>MVLYFIGLGLYDERDITVKGLEIAKKCDYVFAEFYTSLMAGTTLGRIQKLIGKEIRVLSREDVELNFENIVLPLAKENDVAFLTPGDPLVATTHAELRIRAKRAGVESYVIHAPSIYSAVGITGLHIYKFGKSATVAYPEGNWFPTSYYDVIKENAERGLHTLLFLDIKAEKRMYMTANEAMELLLKVEDMKKGGVFTDDTLVVVLARAGSMNPTIRAGYVKDLIREDFGDPPHILIV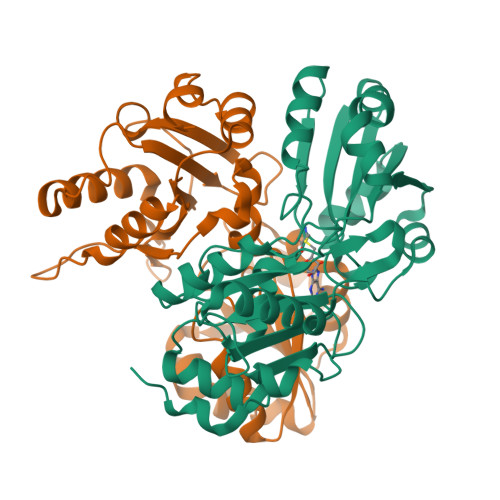PGKLHIVEAEYLVEIAGAPREILRVNV[2x]>MGSSHHHHHHSQDPMVLLHKSTHIFPTDFASVSRAFFNRYPNPYSPHVLSIDTISRNVDQEGNLRTTRLLKKSGKLPTWVKPFLRGITETWIIEVSVVNPANSTMKTYTRNLDHTGIMKVEEYTTYQFDSATSSTIADSRVKFSSGFNMGIKSKVEDWSRTKFDENVKKSRMGMAFVIQKLEEARNPQFLEVLFQGPMGNIMSASFAPECTDLKTKYDSCFNEWYSEKFLKGKSVENECSKQWYAYTTCVNAAL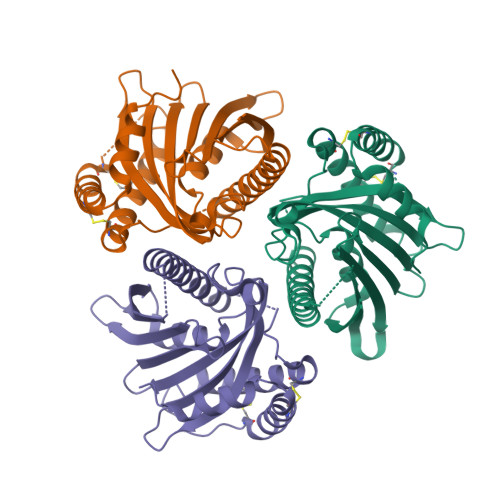VKQGIKPALDEAREEAPFENGGKLKEVDK[3x]> GPGSGQLLFANFNQDNT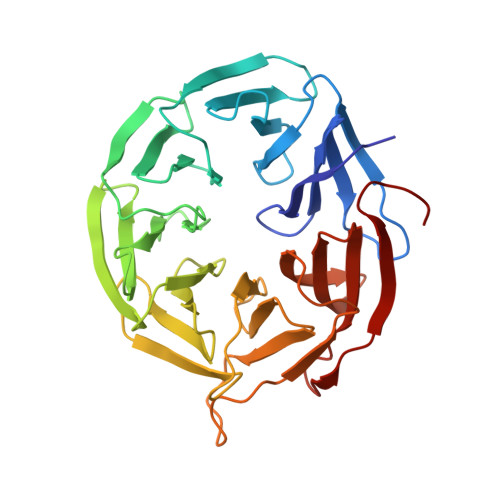SLAVGSKSGYKFFSLSSVDKLEQIYECTDTEDVCIVERLFSSSLVAIVSLKAPRKLKVCHFKKGTEICNYSYSNTILAVKLNRQRLIVCLEESLYIHNIRDMKVLHTIRETPPNPAGLCALSINNDNCYLAYPGSATIGEVQVFDTINLRAANMIPAHDSPLAALAFDASGTKLATASEKGTVIRVFSIPEGQKLFEFRRGVKRCVSICSLAFSMDGMFLSASSNTETVHIFKLETVKEQGRAFATVRLPFCGHKNICSLATIQKIPRLLVGAADGYLYMYNLDPQEGGECALMKQHRLDGSLE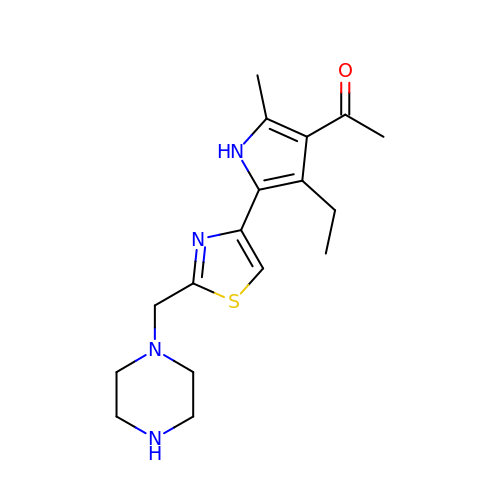1-[4-ethyl-2-methyl-5-[2-(piperazin-1-ylmethyl)-1,3-thiazol-4-yl]-1~{H}-pyrrol-3-yl]ethanone | C17 H24 N4 O S | CWHYBFBVUSCTHI-UHFFFAOYSA-N> AGDMYIVNPDDLQLTFTMEFEVTVTRDGFHKRTISVDNGRPVVVWDGGDKDPKICKICPAVNSINTENIFLDIQKMRLNNLLAQGLWDIQRICVRYVCLFLGFDVVCDVYHTTDRVRAAYTRQTGKIDIQGSGTFSTSDAKGIGTYMIESNVREIKNKWRPTVQKLKQLGYMNETEVEFWYNTTGLTTCVVTSRSNVPFTVELSLNTNSSAIVTEESTVDCQTVTVKAPGSHAQRCYVTSSLGWKGVVTPPSQYRTKRAPVNIHHHHHH;> MGSMELLEYIKREQE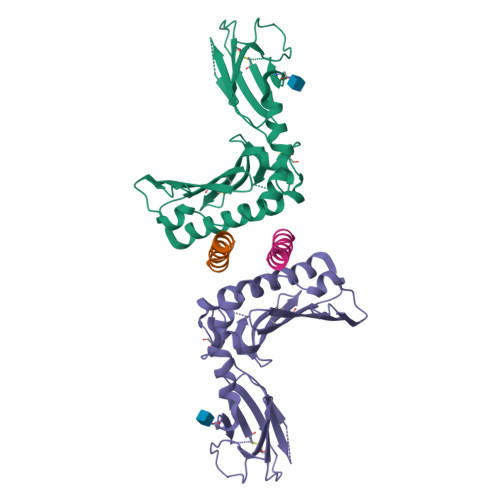RWDSETKSVSDSSRDTGRGVKYWFCYGTKCYYFIMNKTTWSGCKANCQHYSVPIVKIEDEDELKFLQRHVILESYWIGLSYDKKKKEWAWIHNGQSKLDMKIKKMNFTSRGCVFLSKARIEDTDCNTPYYCICGKKLDKFPD> PDVDECALGANP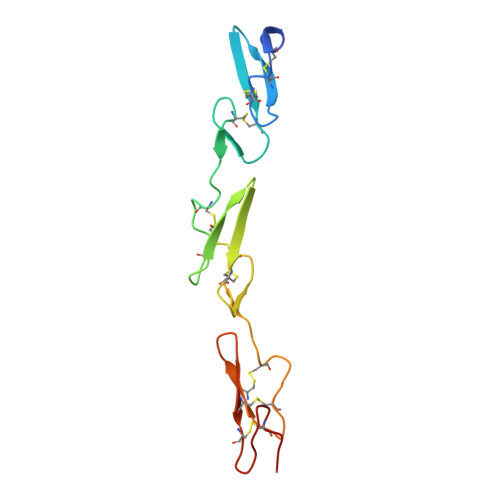CEHAGKCLNTLGSFECQCLQGYTGPRCEIDVNECISNPCQNDATCLDQIGEFQCICMPGYEGVYCEINTDECASSPCLHNGRCVDKINEFLCQCPKGFSGHLCQSG> GPLGSPEFPGSDRNSVDYAQIASGIDTRTTVMIKNIPNKFTQQMLRDYIDVTNKGTYDFLYLRIDFVNKCNVGYAFINFIEPQSIITFGKARVGTQWNVFHSEKICDISYANIQGKDRLIEKFRNSCVMDENPAYRPKIFVSHGPNRGMEEPFPAPNNARRKLRSIASAQQIGLFPPTASKC

Upon meiosis onset, Mmi1 is lured by a ribonucleoprotein (RNP) complex, composed of the nucleocytoplasmic shuttling RNA-binding protein Mei2 and the DSR-containing lncRNA meiRNA, that accumulates in a single nuclear body overlapping the meiRNA-encoding sme2 + gene. Both Mei2 and meiRNA are essential for the assembly of this structure and the completion of sexual differentiation. Interestingly, Mei2 mutants lacking the RRM3 domain (residues 592 to 750, hereafter called RRM3Mei2) failed to accumulate meiotic mRNAs, suggesting that Mei2 RNA-binding activity is required to inhibit Mmi1 function. In this study, we show that the RNA-binding activities of Mmi1 and Mei2 are crucial for their mutual control during mitosis and further identify a lncRNA, termed mamRNA, as a major regulatory and bridging partner for both proteins in the nucleus.

Using isothermal titration calorimetry (ITC) and size exclusion chromatography coupled to multi-angle laser light scattering (SEC-MALLS), we found that RRM3Mei2 tightly interacts with a poly-U15 in a 1:1 stoichiometry. Given the interaction of a guanine (G11) with Sxl F170, which corresponds to Mei2 F644 that is essential for Mei2 function in vivo, we also tested the influence of one (U7GU7) or two (U6GGU7) Gs in a poly-U15 oligonucleotide and observed a considerable increase of Mei2 binding to these RNAs. We next solved the crystal structure of RRM3Mei2 bound to the GCUUUUUGUUCG 12-mer. The RRM3Mei2–RNA complex revealed that F644 and F634 side chains form π–π stacking interactions with U7 and G8, respectively. As revealed by the PISA server, several Mei2 residues also form specific hydrogen bonds with U4 to G8, rationalizing the stronger affinity for U7GU7 than for poly-U15. U4 binding pocket is solvent exposed and hence any nucleotide may fit in it. Importantly, Mei2F644A protein levels were roughly 10-fold more abundant than wild-type Mei2. Although mei2-F644A mRNAs were also increased by 3-fold when compared to wild-type mei2 + transcripts, these data strongly suggest that Mei2 RNA-binding activity is required for its own downregulation. Further, expression of the Mei2-F644A mutant did not lead to the accumulation of meiotic mRNAs in mot2∆ mei2∆ cells, consistent with RRM3Mei2 RNA-binding activity being also required for Mmi1 inactivation.> MVIGLSTGSDDDDVEVIGGVDPRLIAVQENDSDESSLTDLVEQPAKVMRIGTMIKQLLEEVRAAPLDEASRNRLRDIHATSIRELEDGLAPELREELDRLTLPFNEDAVPSDAELRIAQAQLVGWLEGLFHGIQTALFAQQMAARAQLQQMRQG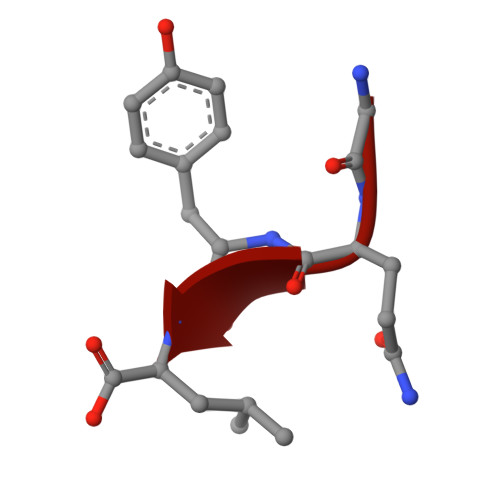ALPPGVGKSGQHGHGTGQYL>[4x]GSESSSQAVVVAIDAKRVDGEFMVFTYSGKKNTGILL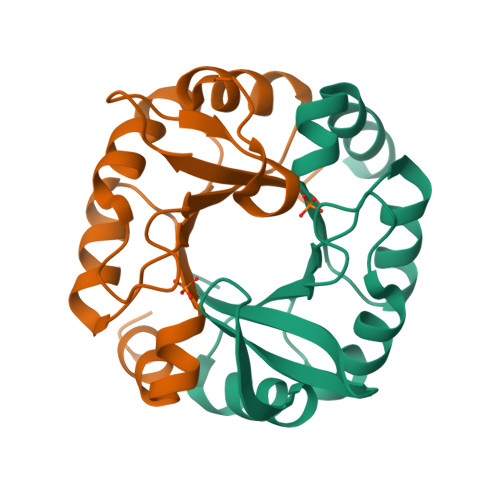RDWVVEVEKRGAGEILLTSIDRDGTKSGYDTEMIRFVRPLTTLPIIASGGAGKMEHFLEAFLRGADKVSINTAAVENPSLITQIAQTFG>GSMNVILSIDQSTQSTKVFFYDEELNIVHSNNLNHEQKCLKPGWYEHDPIEIMTNLYNLMNEGIKVLKDKYTSVIIKCIGITNQRETVIIWDRITGKPLYNAIVWLDTRVEELVTEFSAKYNNNDIQKKTGTYFNTYFSAFKILWLIQNNPEIKQKIDDGTAVIGNINTWLIFNLTKGNCYTDVTNASRTLLMDINTLQWDEKMCKIFNITNMSVLPEIKSNCSNFGLVKSEHVPDYLNIPITGCIGDQQSACIGQAIFDEGEAKCTYGTGVFLLINTGEKVVYSTCGLITTICYKFNDNDKPKYALEGSIGTAGSGVSWLLKNKLIDDPSEASDIMEKCENTTGVIFVPA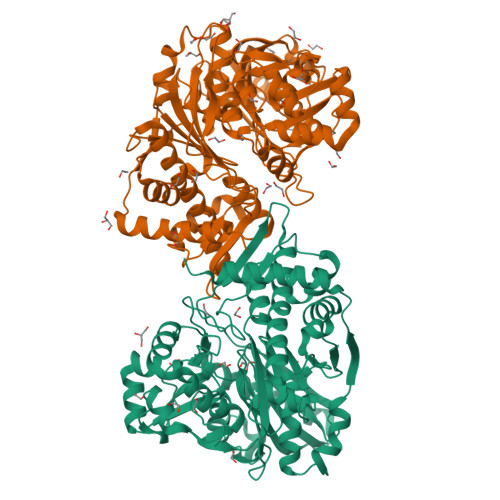FSGLYAPRWRSDARASIYGMTFNTERSHIVRALLEGIAFQLNEIVDSLTSDMGIEMLHVLRCDGGMTKNKPFMQFNSDIINTKIEVSKYKEVTSLGAAVLAGLEVKIWDSLDSVKSLLRRSDAVFHSKMDDKKRKKKTSEWNKAVERTLIQL[4x]4-[(2-phenylimidazo[1,2-a]pyridin-3-yl)amino]benzene-1,2-dicarboxylic 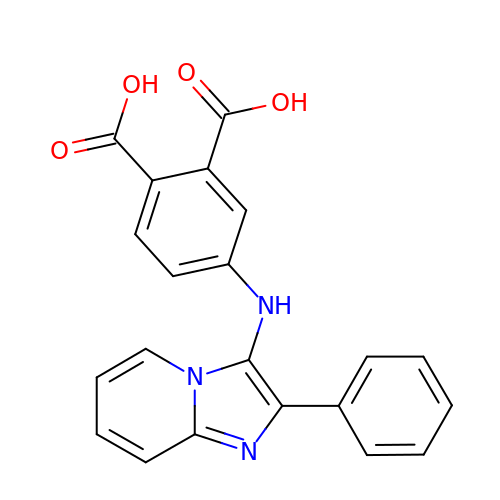acid | C21 H15 N3 O4 | RSBAGHOCQVUFFP-UHFFFAOYSA-N> MVFGQLYALFIFTLSCCISKTVQADSSKESSSFISFDKESNWDTISTISSTADVISSVDSAIAVFEFDNFSLLDNLMIDEEYPFFNRFFANDVSLTVHDDSPLNISQSLSPIMEQFTVDELPESASDLLYEYSLDDKSIVLFKFTSDAYDLKKLDEFIDSCLSFLEDKSGDNLTVVINSLGWAFE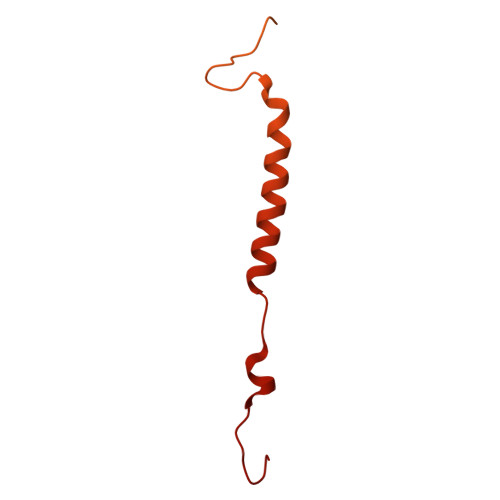DEDGDDEYATEETLSHHDNNKGKEGDDDILSSIWTEGLLMCLIVSALLLFILIVALSWISNLDITYGALEKSTNPIKKNN> ANPLYQKHIISINDLSRDDLNLVLATAAKLKANPQP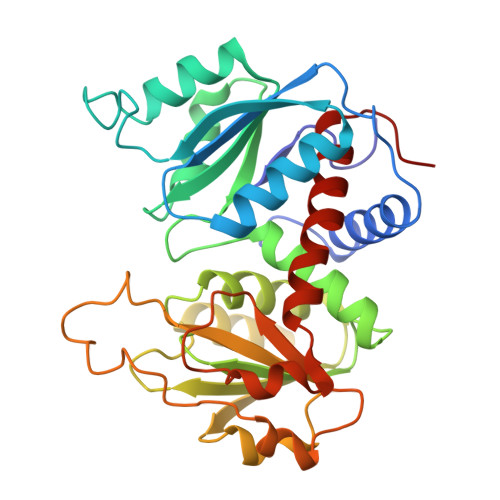ELLKHKVIASCFFEASTATRLSFQTSMHRLGASVVGFSDSANTSLGKKGETLADTISVISTYVDAIVMRHPQEGAARLATEFSGNVPVLNAGDGSNQHPTQTLLDLFTIQQTEGRLDNLHVAMVGDLKYGRTVHSLTQALAKFDGNRFYFIAPDALAMPEYILDMLDEKGIAWSLHSSIEEVMAEVDILYMTRVQKERLDPSEYANVKAQFVLRASDLHNAKANMKVLHPLPRVDEIATDVDKTPHAWYFQQAGNGIFARQALLALVLNRDLVL>MPVFTASFQCVTLFGQPASAADAQPLLQGQRPFLHLHARRRRPCGPMLISKSPPYPASEETREWEADGQHEHTDELRETTTTMIDGIRTALRSIGEGEISISAYDTSLVALLKRLDGGDGPQFPSTIDWIVQNQLPDGSWGDASFFMMGDRIMSTLACVVALKSWNIHTDKCERGLLFIQENMWRLAHEEEDWMLVGFEIALPSLLDMAKDLDLDIPYDEPALKAIYAERERKLAKIPRDVLHSMPTTLLHSLEGMVDLDWEKLLKLRCLDGSFHCSPASTATAFQQTGDQKCFEYLDGIVKKFNGGVPCIYPLDVYERLWAVDRLTRLGISRHFTSEIEDCLDYIFRNWTPDGLAHTKNCPVKDIDDTAMGFRLLRLYGYQVDPCVLKKFEKDGKFFCLHGESNPSSVTPMYNTYRASQLKFPGDDGVLGRAEVFCRSFLQDRRGSNRMKDKWAIAKDIPGEVEYAMDYPWKASLPRIETRLYLDQYGGSGDVWIGKVLHRMTLFCNDLYLKAAKADFSNFQKECRVELNGLRRWYLRSNLEKFGGTDPQTTLMTSYFLASANIFEANRAAERLGWARVALLADAVSSHFRRIGGPKNSTSNLEELISLVPFDDAYSGSLREAWKQWLMAWTAKESSQESIEGDTAILLVRAIEIFGGRHVLTGQRPDLWEYSQLEQLTSSICCKLSRRVLAQENGESTEKVEEIDQQVDLEMQELTRRVLQGCSAINRLTRETFLHVVKSFCYVAYCSPETIDSHIDKVIFQDVIEFHHHHHH[2x]

The large superfamily of labdane-related diterpenoids is defined by the cyclization of linear geranylgeranyl pyrophosphate (GGPP), catalyzed by copalyl diphosphate synthases (CPSs) to form the basic decalin core, the copalyl diphosphates (CPPs). Here, we used X-ray crystallography and cryo-EM methods to describe different oligomeric structures of a syn-copalyl diphosphate synthase from Oryza sativa (OsCyc1), and provided a cryo-EM structure of OsCyc1D367A mutant in complex with the substrate GGPP. The structure of monomer OsCyc1 consists of an αβγ domain and a catalytic center located between the β and γ domains. OsCyc1 catalyzes GGPP to form syn-CPP, in which new bonds form between C6 and C11, as well as between C10 and C15.

To elucidate the oligomer states and the interaction mode of OsCyc1, we determined the cryo-EM structure of OsCyc1 and finally solved three OsCyc1 structures in dimer, tetramer and hexamer forms, at a resolution of 7.9 Å, 3.5 Å and 3.7 Å, respectively. The dimer is composed of protomer A and protomer B, and the dimerization interface involves their α domains. The interactions in the dimer assembly of protomers/chains A and B occur symmetrically in α domain helices α22, α23, α24 and α25. Residues S674 and E677 are both located in the original dimer interface and form hydrogen bonds. The S674A/E677A mutant form exhibited the highest relative enzyme activity, comparable to that of WT, and showed a lagging peak position in the size exclusion chromatograph, indicating that S674A/E677A is present in a state of lower oligomerization.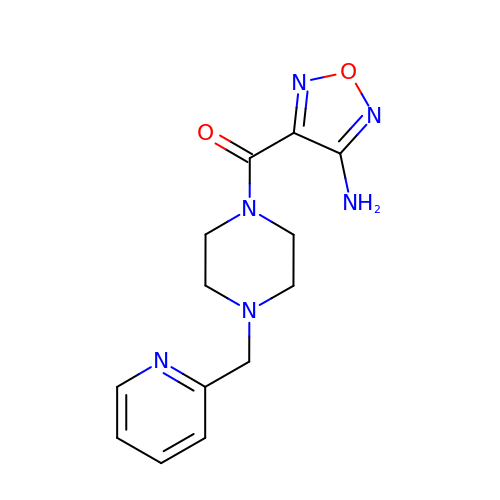(4-amino-1,2,5-oxadiazol-3-yl)[4-(pyridin-2-ylmethyl)piperazin-1-yl]methanone | C13 H16 N6 O2 | IBQSBIBAFXRXMH-UHFFFAOYSA-N>MELIRIAMRKDLENDKSLMSKWAAVAGLKNPNPLYDFLNHDGKTFSEFNSIVNIVKTHYPDQEYELMENYCLLLDPNTKAARSALEYADANSFNTLTDKLVEKMSIASNLKSKEYGKIYEIHRKLSRGEIDVLEASKNIGKYRIKTDEMNIFSKMIPMYDYLSKGNFSPMKSLLKQIDLNDIKENNYLKKSFETRIYVLLSNIYLNENELELSRKYAEKAIKSTDTKRFLVFSYLTIGTSYIFSDYALSKQNYLSGYEIAKGNSVFEEFFKRNLSFLNNFWNKENPWINYDSNAVTDVQEVIFELINQKKLERALTLLKSLERKKQNENDLGFHYYLEGLITNDKEAFYKSVEYFKLSQDKLFIKMPLIKLESLGENPRLLK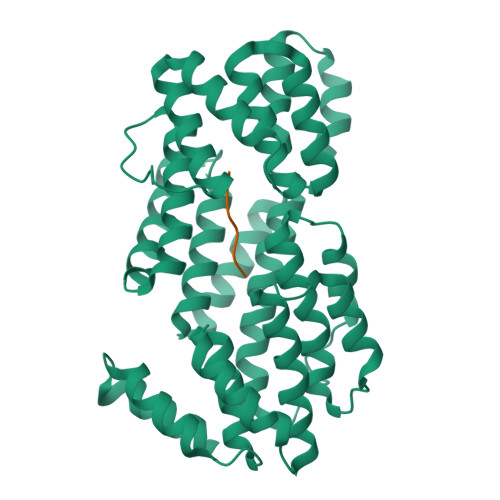IISM[4x];>GVVRGA[4x]>[2x]SWVWNQFFVLEEYM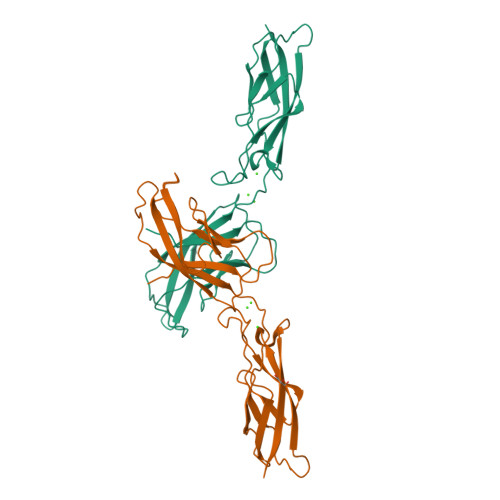GSDPLYVGKLHSDVDKGDGSIKYILSGEGASSIFIIDENTGDIHATKRLDREEQAYYTLRAQALDRLTNKPVEPESEFVIKIQDINDNEPKFLDGPYTAGVPEMSPVGTSVVQVTATDADDPTYGNSARVVYSILQGQPYFSVEPKTGVIKTALPNMDREAKDQYLLVIQAKDMVGQNGGLSGTTSVTVTLTD>MRGSHHHHHHGSAKNVVLDHDGNLDDFVAMVLLASNTEKVRLIGALCTDADCFVENGFNVTGKIMCLMHNNMNLPLFPIGKSAATAVNPFPKEWRCLAKNMDDMPILNIPENVELWDKIKAENEKYEGQQLLADLVMNSEEKVTICVTGPLSNVAWCIDKYGEKFTSKVEECVIMGGAVDVRGNVFLPSTDGTAEWNIYWDPASAKTVFGCPGLRRIMFSLDSTNTVPVRSPYVQRFGEQTNFLLSILVGTMWAMCTHCELLRDG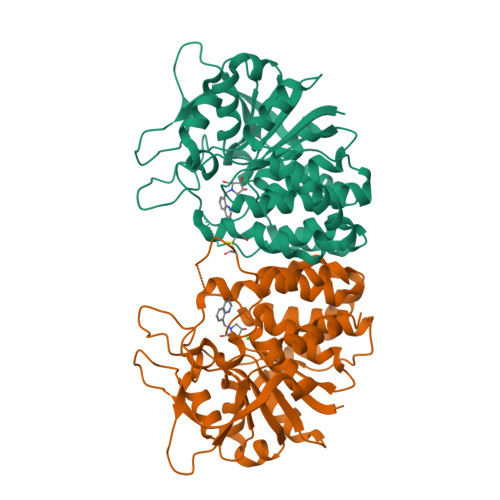DGYYAWDALTAAYVVDQKVANVDPVPIDVVVDKQPNEGATVRTDAENYPLTFVARNPEAEFFLDMLLRSARAC[2x]>[2x]MPKRGKKGAVAEDGDELRTEPEAKKSKTAAKKNDKEAAGEGPALYEDPPDQKTSPSGKPATLKICSWNVDGLRA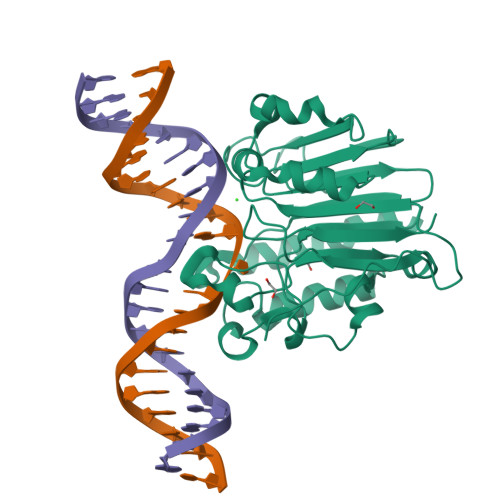WIKKKGLDWVKEEAPDILCLQQTKCSENKLPAELQELPGLSHQYWSAPSDKEGYSGVGLLSRQCPLKVSYGIGDEEHDQEGRVIVAEFDSFVLVTAYVPNAGRGLVRLEYRQRWDEAFRKFLKGLASRKPLVLCGNLNVAHEEIDLRNPKGNKKNAGFTPQERQGFGELLQAVPLADSFRHLYPNTPYAYTFWTYMMNARSKNVGWRLDYFLLSHSLLPALCDSKIRSKALGSDHCPITLYLAL>[2x]HHHHHHFNLPPGNYKKPCLLYCSNGGHFLRILPDGTVDGTRDRSDQHIQLQLSAESVGEVYIKSTETGQYLAM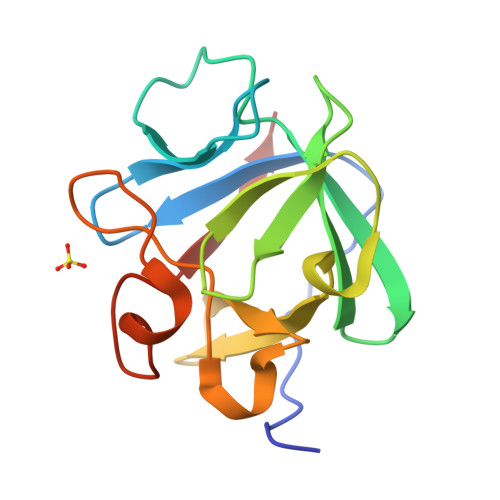DTDGLLYGSQTPNEECLFLERLEENHYNTYISKKHAEKNWFVGLKKNGSVKRGPRTHYGQKAILFLPLPVSSD> MTENILRKSDEEIQKEITARVKALESMLIEQGILTTSMIDRMAEIYENEVGPHLGAKVVVKAWTDPEFKKRLLADGTEACKELGIGGLQGEDMMWVENTDEVHHVVVCTLCSCYPWPVLGLPPNWFKEPQYRSRVVREPRQLLKEEFGFEVPPSKEIKVWDSS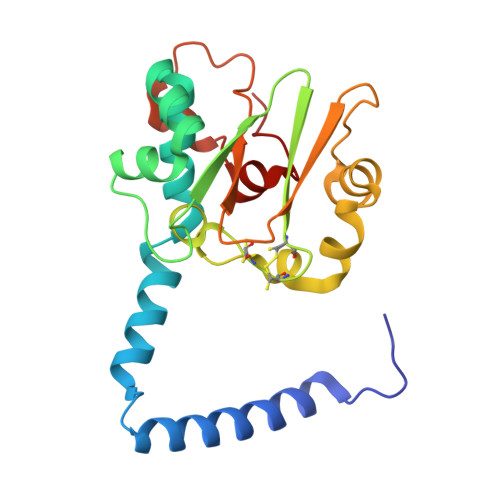SEMRFVVLPQRPAGTDGWSEEELATLVTRESMIGVEPAKAV> MIRRSCALLSSSWRDHGISYLKYLNVCTETLHST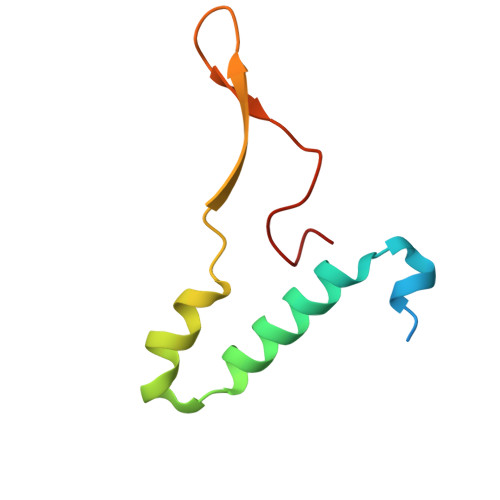VKESRRAKYERWSKPCYTAQRPDGAGGQETIDKVPIHTKDY> AHHHHHHGSRELVEIIKGIGIEGAKEVEEKVDRQFYALQYLFRHQDPEMFIKLVIANSLVSYQLTGRGEDWWWEFARYFSGREVDSIWKAYGEFLPKSKNNRRLIEAKLNRIRKVEGFLSTLTLKDLEGYYKNMKMLWKALIKIMGSREDSKTIVFTVKMFGYASRIAFSRFIPYPMEIPI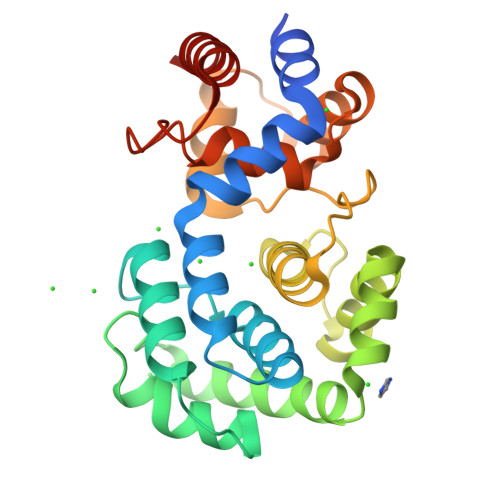PEDLRIKSVTSKLTQEKPTKFWMKIGQESGVPPLHIDSLIWPLLGNADLTPLDIELRNKLMKLTELLGL> MSPSMQQRTDLPAKDSSKSELQLAREQLHVSVVPKSLPCREREFENIYAFLEGKIQDQCGGCMYVSGVPGTGKTATVTGVIRTLQRMAKQNELPAFEYLEINGMRLTEPRQAYVQI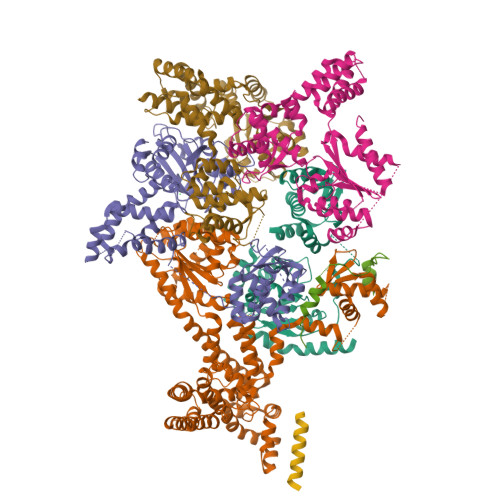YKQLTGKTVSWEQAHALLEKRFTTPAPRRVTTVLLVDELDILCNRRQDVVYNLLDWPTKSAAKLVVVTIANTMDLPERLLMGKVTSRLGLTRLTFQPYSHKQLQEIVTARLGGSETFKGEAVQLVARKVAAVSGDARRALDICRRATEIADTAAVKCVTMLHVQQALAEMIASAKVQAIRNCSRMEQIFLQAIAAEVTRTGVEETTFMGVYQQVETIAAFMGVTFPPPGRALRLCSKLGAERLIISEHSRNDLFQKILLNVSADDIHYALRVEEMVN;> MQSARAKKSNEFVPESDGYFHSHASSKILTSDHTLDRLKNPRLAADRVFSLLSEIKTSAEHEGSINAIMEEYRSYFPKWMCILNEGFNILLYGLGSKHQLLQSFHREVLHKQTVLVVNGFFPSLTIKDMLDSITSDILDAGISPANPHEAVDMIEEEFALIPETHLFLIVHNLDGAMLRNVKAQAILSRLARIPNIHLLASIDHINTPLLWDQGKLCSFNFSWWDCTTMLPYTNETAFENSLLVQNSGELALSSMRSVFSSLTTNSRGIYMLIVKYQLKNKGNATYQGMPFRDLYSSCREAFLVSSDLALRAQLTEFLDHKLVKSKRSVDGSEQLTIPIDGALLQQFLEEQEKK;> MQPFYEEYRKAWNQINDHIADLQHRSYARTLEQLVDFVVGQAERDTPDEVLPTAALLTGINQPDHLSQFTALTQRLHAQRAAMVCVLQSRDCATLKAAVETLVFGLVEDNAEVEQMEDEDEDEDGAERDRKRLRRSQCTMKQLKSWYTNNFDSEQKRRQLVVILPDFECFNASVLQDLILILSAHCGSLPFVLVLGVATAMTAVHGTLPYHVSSKIRLRVFQTQAAPTGLNEVLDKVLLSPKYAFHLSGKTFKFLTHIFLYYDFSIHGFIQGFKYCLMEHFFGGNAFALCTDYSKALGRIKQLTHEDMETIRRLPSFRPYVEQINDCKRIIAVLTDDDYLKKKLPQLLRDCLLHFLLFRCSLEFLTELVGDLPRCPLGKLRRELYVNCLNRAIISTPEYKECLQMLSFLSKDEFVAKVNRALERTEQFLVEEIAPLELGEACTAVLRPKLEAIRLAVDEVVKATMATITTTSPNETRQATDHLTPVASRQELKDQLLQRSKEDKMRHQLNTPTTQFGRALQKTLQLIETQIVQDHLRALQDAPPIHELFVFSDIATVRRNIIGAPRAALHTALNNPHFYMQCKCCELQDQSLLVGTLPDLSVVYKLHLECGRMINLFDWLQAFRSVVSDSDHEEVAQEQIDPQIQARFTRAVAELQFLGYIKMSKRKTDHATRLTW;> MPEADRELVSIRRFLKERLQRDYTTLRGYAKERSNVRLLLQRTAEMGESNSLLLLGPRGSGKTTLINSVLADLLPNKSFGENTLIVHLDGNLHTDDRVALKSITVQMQLENAADGKVFGSFAENLAFLLQCLKAGGKHSKSVIFILEEFDLFCAHHNQTLLYNLFDVSQSAQAPICVLGVTCRLDVIELLEKRVKSRFSHRQVFLFPSLRRFEDYVDLCRDLLSLPTGNSLLLAAEKIYNLQNIQSGALYFSRNHFDPGEYGFSPRLRDAWNKQICKVLATQQARSTLQALHDFDISEAYLKNFLFRLVAHLRPQSPHITAEKMAAVGSQFEGDDKIELLCGLSVLELCLIIAIKHHSQIYDRDSFNFEIIYARFSKFAKVSTTMQAVERSIVLKAFEHLRIAELIMPLTGGAGGGVGKVQKEFEMHKLALTYSQIHHCMQRYQALPTEVAQWAQSSLI;> MEAICSSLEPLFPCREAAIETLGELIGDSSETYPSAIYLFGHSGTGKTALTRAFLKECGKRQNVRTAHLNAIECYTTKIMLEILLDSLAPDQGDALKVDNMLDFVEQLRRQAATRVEDQGFLIAVDNAERLRDMDANVLPVLLRLQELTNLNLCVILLSQLPFEKFYNKTGLSEIVCLHLAQYNKAETQRILGSDFQQVRNQLLEQFAQDKKRLEICQEAVTEDFYNNYLNLFLSVFYKACRDVPELQLTARKCLSTYLEPVLDGTVDATDISRLWRHIAGPLRSALTQIYMRIEKPAEEVEDFTAIEDQSVRKLAQSLELPYYAKFLLIAAFLASHNAAKQDKRLFVKHHGKQRKRMQTVNARAKTTEKMSTTLGPKSFSIDRLLAIFYAILEEKVGLTCNLLSQISTLVHLNLLSFVSGEQNIMEGSARLQCTIGLEFVLQIGKVVGFNVRQYLCDFM;> MKESKVPSSTDMEGKLKENQNENIKGHEAKKAHKPPPEDYEIWKARMLAKAQAKLKELEASQSHMDSQLLEA> NALPTWWKQAVFYQVYPRSFKDTNGDGIGDLNGIIENLDYLKKLGIDAIWINPHYDSPNTDNGYDIRDYRKIMKEYGTMEDFDRLISEMKKRNMRLMIDIVINHTSDQHAWFVQSKSGKNNPYRDYYFWRDGKDGHAPNNYPSFFGGSAWEKDDKSGQYYLHYFAKQQPDLNWDNPKVRQDLYDMLRFWLDKGVSGLRFDTVATYSKIPNFPDLSQQQLKNFAEEYTKGPKIHDYVNEMNREVLSHYDIATAGQIFGVPLDKSIKFFDRRRNELNIAFTFDLIRLDRDADERWRRKDWTLSQFRKIVDKVDQTAGEYGWNAFFLDNHDNPRAVSHFGDDRPQWREHAAKALATLTLTQRATPFIYQGSELGMTNYPFKKIDDFDDVEVKGFWQDYVETGKVKAEEFLQNVRQTSRDNSRTPFQWDASKNAGFTSGTPWLKINPNYKEINSADQINNPNSVFNYYRKLINIRHDIPALTYGSYIDLDPDNNSVYAYTRTLGAEKYLVVINFKEEVMHYTLPGDLSINKVITENNSHTIVNKNDRQLRLEPWQSGIYKLNP

SIases, classified as glycoside hydrolase family 13 (GH13) enzymes, catalyze the isomerization of sucrose to produce isomaltulose and trehalulose as primary products and D-glucose and D-fructose as by-products. NX-5 (named NX-5 in this work) that predominantly produces isomaltulose (~87%). Similar to other GH13 family enzymes, the NX-5 molecule is composed of three domains: the N-domain (residues 42-145 and 216-520), the sub-domain (residues 146-215), and the C-domain (residues 521-600). Among them, residues Asp102, His145, Arg239, His368, Asp369, Glu428, and Arg456 are responsible for sucrose binding and residues Asp241 (the nucleophile) and Glu295 (the acid catalyst) are crucial for sucrose hydrolysis for PalI, MutB, and SmuA.

To investigate the mechanism of substrate binding and sucrose isomerization, we determined the crystal structure of the inactive E295Q mutant in complex with the substrate sucrose at 1.70 Å resolution. In the structure, the sucrose molecule was deeply bound in the active site with the glucosyl ring at subsite -1 and fructosyl moiety at subsite +1. The glucosyl ring of sucrose interacts with a water molecule and eight residues of NX-5 (Asp102, His145, Arg239, Asp241, Gln295, His368, Asp369, and Arg456) via a hydrogen-bond network as well as through π-π stacking with Tyr105 and Phe205. The fructosyl moiety of sucrose binds to NX-5 through direct hydrogen bonds with Gln295, Asp369 and Glu428, hydrophobic interactions with Phe297, and hydrogen bonds between 1’-OH, 3’-OH, 4’-OH, 6’-OH and four water molecules. Therefore, the fructosyl moiety of sucrose has fewer interactions with the active site pocket, which should allow it to exit easily after sucrose hydrolysis and undergo tautomerization resulting in trehalulose production. Upon sucrose binding, the phenyl rings of Phe297 and Phe321 were forced to move away from the substrate. Substrate binding also pushed the side chain of Arg325 towards Arg328. Glu428 is involved in a 2.39 Å hydrogen bond to the 6’-OH of the fructosyl moiety, which induces the O6’-C6’ bond to rotate 98.9°. The most prominent structural differences between NX-5 and MutB occur in the catalytic325RLDRD329 motif and its adjacent 10-residue loop (residues 330-339). The conformation of the 10-residue loop (residues 330-339) in NX-5 was remarkably different from that of the corresponding loop (residues 289-297) in MutB.> MMKKQIINKKDLLGLGPNSKLIKDYKKQWTTLSKIQEETLIGNILGDVYIKKLKRNKHFLLQFEWKNKAYIEHIVRVFDEYVISPPTLYERKNHLGNKVITWRAQTFEHKAFDKLGYYFMENHKKIIKPDLVLNYITERSLAYWFMDDGGKWDYNKKTKNKSLVLHTQGFKKEEVEILINDLNIKFNLNCSIKFNKNKPIIYIPNKDYELFYNLVNPY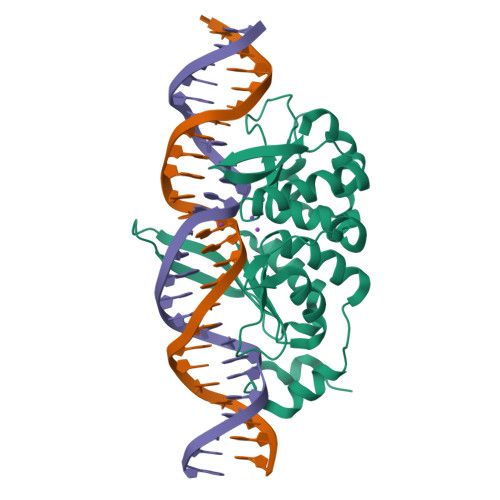IIPEMKYKLLFNV1-[4-(trifluoromethoxy)phenyl]methanamine 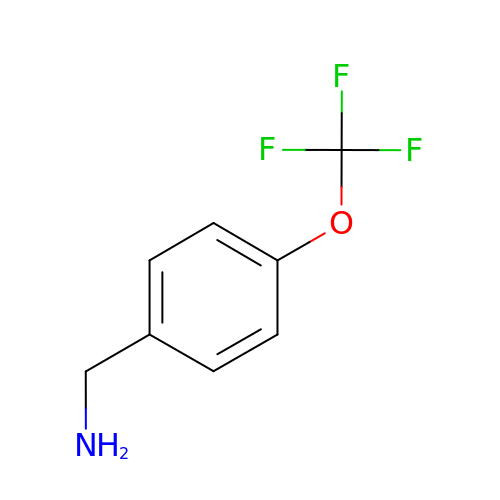| C8 H8 F3 N O | DBGROTRFYBSUTR-UHFFFAOYSA-N> 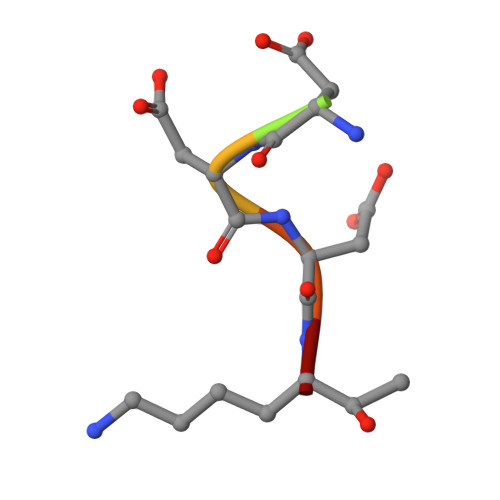VDDDDKX> GPSRGAQNSISWEVQRFDGWYNNLMEHRWGSKGSRLQRLVPASYADGVYQPLKEPYLPNPRHLSNRVMRGSAGQPSLRNRTVLGVFFGYHVLSDLVSVETPGCPAEFLNIYIPHGDPVFDPDKRGNVVLPFQRSRWDRNTGQSPSNPRDQSNQVTGWLDGSAIYGSSHSWSDTLRSFSGGQLASGPDPAFPSDSQSSLLMWMAPDPSTGQGGPRGVYAFGAQRGNREPFLQALGLLWFRYHNLCARKLAQEHPHWGDEELFQHARKRVIATYQNIAMYEWLPSFLKQTPPEYPGYRPFLDPSISPEFVVASEQFLSTMVPSGVYMRNASCHFQGIPSHNSSVSGALRVCNSYWSREHPKLQRAEDVDALLLGMASQIAEREDHVVVEDMQDFWPGPLKFSRTDYLASCLQRGRDLGLPSYTKAREALGLSPISHWQDINPALSRSNGTVLEATAALYNQDLSRLELLPGGLLE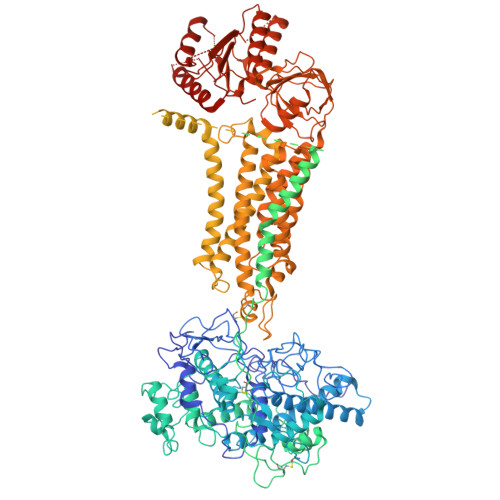SHGDPGPLFSTIVLDQFVRLRDGDRYWFENTRNGLFSKEEIAEIRNTSLRDILVAVTNVDPSALQPNVFFWLAGDPCPQPSQLSAKGLPACAPLFIRDYFEGSGFGFGLTIGTLCCFPLVSLLSAWIVARLRKRNFKRLQRQDRQSIMSEKLVGGVEALEWQGRNEPCRPVLVHLQPGQIRVVDGRLTVLRTIQLRPPQQVNLILSSNRGRRTLLLKIPKEYDLVLLFNMEEERQALVENVRGALKENGLSFQEWELREQELMRAAVTRQQRGHLLETFFRHLFSQVLDINQADAGTLPLDSSTKVREALTCELSRAEFADSLGLKPQDMFVESMFSLADKDGNGYLSFREFLDILVVFMKGSPEEKSRLMFRMYDFDGNGLISKDEFIRMLRSFIEISNNCLSKAQLAEVVESMFRESGFQDKEELTWEDFHFMLRDHDSDLRFTQLCVKGVEVPEVIKNLCRRASYISQEKICPSPRMSAHCARNNMKTASSPQRLQCPMDTDPPQEIRRRFGKKVTSFQPLLFTEAHREKFQRSRRHQTVQQFKRFIENYRRHIGCVAVFYTITGALFLERAYYYAFAAHHSGITDTTRVGIILSRGTAASISFMFSYILLTMCRNLITFLRETFLNRYIPFDAAVDFHRLIASTAIILTVLHSAGHVVNVYLFSISPLSVLSCLFPGLFHDDGSEFPQKYYWWFFQTVPGLTGVLLLLALAIMYVFASHHFRRRSFRGFWLTHHLYIFLYILLIIHGSFALIQMPRFHIFFLVPAIIYVGDKLVSLSRKKVEISVVKAELLPSGVTHLRFQRPQGFEYKSGQWVRIACLALGTTEYHPFTLTSAPHEDTLSLHIRAAGPWTTRLREIYSPPTGDTCARYPKLYLDGPFGEGHQEWHKFEVSVLVGGGIGVTPFASILKDLVFKSSVSCQVFCKKIYFIWVTRTQRQFEWLADIIREVEENDRQDLVSVHIYITQLAEKFDLRTTMLYICERHFQKVLNRSLFTGLRSITHFGRPPFEPFFNSLQEVHPQVRKIGVFSCGPPGMTKNVEKACQLINRQDRTHFSHHYENF>MAKKTPPLVFYWIPWFGSAASYGQQPYEFFESCRQKYGDVFSFMLLGKIMTVYLGPKGHEFVFNAKLSDVSAEEAYKHLTTPVFGTGVIYDCPNSRLMEQKKFAKFALTTDSFKRYVPKIREEILNYFVTDESFKLKEKTHGVANVMKTQPEITIFTASRSLFGDEMRRIFDRSFAQLYSDLDKGFTPINFVFPNLPLPHYWRRDAAQKKISATYMKEIKLRRERGDIDPNRDLIDSLLIHSTYKDGVKMTDQEIANLLIGILMGGQHTSASTSAWFLLHLGEKPHLQDVIYQEVVELLKEKGGDLNDLTYEDLQKLPSVNNTIKETLRMHMPLHSIFRKVTNPLRIPETNYIVPKGHYVLVSPGYAHTSERYFDNPEDFDPTRWD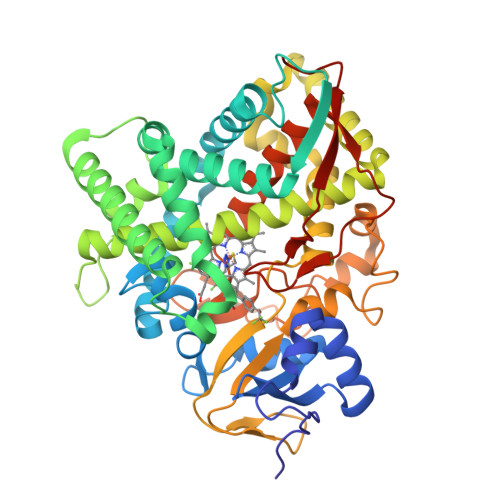TAAAKANSVSFNSSDEVDYGFGKVSKGVSSPYLPFGGGRHRCIGEQFAYVQLGTILTTFVYNLRWTIDGYKVPDPDYSSMVVLPTEPAEIIWEKRETCMFHHHH[2x]> MAKKTSSKGKLPPGPSPLPVLGNLLQMDRKGLLRSFLRLREKYGDVFTVYLGSRPVVVLCGTDAIREALVDQAEAFSGRGKIAVVDPIFQGYGVIFANGERWRALRRFSLATMRDFGMGKRSVEERIQEEARCLVEELRKSKGALLDNTLLFHSITSNIICSIVFGKRFDYKDPVFLRLLDLWFQSFSLISSFSSQVFELFSGFLKYFPGTHRQIYRNLQEINTFIGQSVEKHRATLDPSNPRDFIDVYLLRMEKDKSDPSSEFHHQNLILTVLSLFFAGTETTSTTLRYGFLLMLKYPHVTERVQKEIEQVIGSHRPPALDDRAKMPYT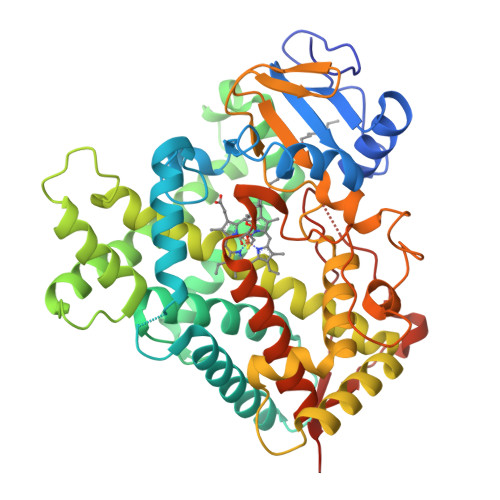DAVIHEIQRLGDLIPFGVPHTVTKDTQFRGYVIPKNTEVFPVLSSALHDPRYFETPNTFNPGHFLDANGALKRNEGFMPFSLGKRICLGEGIARTELFLFFTTILQNFSIASPVPPEDIDLTPRESGVGNVPPSYQIRFLARHHHHHH>[2x]MSQTHKHAIPANIADRCLINPEQYETKYKQSINDPDTFWGEQGKILDWITPYQKVKNTSFAPGNVSIKWYEDGTLNLAANCLDRHLQENGDRTAIIWEGDDTSQSKHISYRELHRDVCRFANTLLDLGIKKGDVVAIYMPMVPEAAVAMLACARIGAVHSVIFGGFSPEAVAGRIIDSSSRLVITADEGVRAGRSIPLKKNVDDALKNPNVTSVEHVIVLKRTGSDIDWQEGRDLWWRDLIEKASPEHQPEAMNAEDPLFILYTSGSTGKPKGVLHTTGGYLVYAATTFKYVFDYHPGDIYWCTADVGWVTGHSYLLYGPLACGATTLMFEGVPNWPTPARM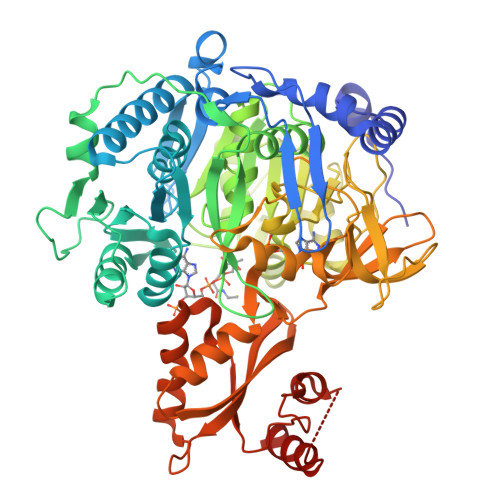CQVVDKHQVNILYTAPTAIRALMAEGDKAIEGTDRSSLRILGSAGEPINPEAWEWYWKKIGKEKCPVVDTWWQTETGGFMITPLPGAIELKAGSATRPFFGVQPALVDNEGHPQEGATEGNLVITDSWPGQARTLFGDHERFEQTYFSTFKNMYFSGDGARRDEDGYYWITGRVDDVLNVSGHRLGTAEIESALVAHPKIAEAAVVGIPHAIKGQAIYAYVTLNHGEEPSPELYAEVRNWVRKEIGPLATPDVLHWTDSLPKTRSGKIMRRILRKIAAGDTSNLGDTSTLADPGVVEKLLEEKQAIAMPS>MNTIAWLGRLVIERIRGIGVAALMLLQIIFSLPSAGGFGRFVYQMHRVGVMSLLIITVSGLFIGLVLGLQGYSILVNVGSESMLGTMVSLTLLRELAPVVAALLFAGRAGSALTAEIGSMKQSEQLASMEMIGVDPLKQIVSPRLWAGIVSLPMLTVIFAAIGIVGGKLVGVDFLGVDEGSFWSGMQNNVQFGHDVVNGIIKSIVFALLCTWIAVFQGYACDPTPEGIATAMTRTVVYSSLCVLGFDFVLTAVMFGGI[2x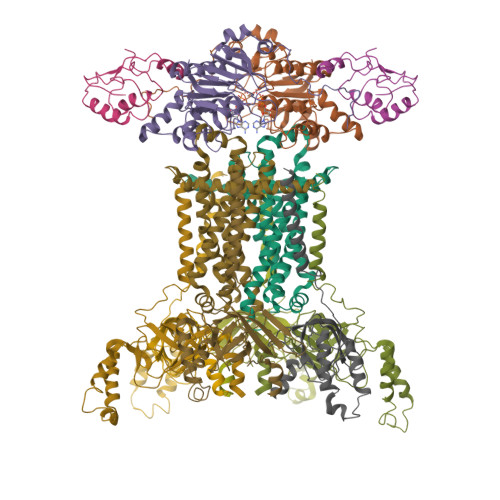];>MMNNKTPLSTQSLIEVKNLSFNRGERVIYDNISLNIRRGQITAIMGPSGTGKTTLLRLIGGQLVPDQGEVLLDGKDIAQMSRQELFAARARMGMLFQSGALFTDMSVYENVAFPIRAHTKLSENLIAELVALKLESVGLRGTEQLMPTELSGGMNRRVALARAIALDPDLIMYDEPFAGQDPIVKGVLTRLIRSLREALDLTTIIVSHDVPETLSIADYIYVVAEGKIQGEGTPEELQAYASPFVKQFLTGSAEGPVEYQFSHQAYLDNEVRP[2x];>[2x]VVQYLNQELVVSGKIDFENAEQQYQAGLAIIKKQTSFPLIVDLKQLEHGNTLALAVLVQWLRQTPQKSGLHFKNVPEKMLKIIQACHLQEDLHLVLEHHHHHH;>MKSRTSELAVGIFVIIFGIALFFLAMKVSGLVGTNLSDGYTMKAQFDNVNGLKPRAKVTMSGVTIGRVDSITLDPVTRLATVTFDLDGKLTSFNAEQLKEVQKNALDELRYSSDYTQATPAQQKTMEQQLISNMNSITSIDEDAYIMVATNGLLGEKYLKIVPGGGLNYLKRGDTISNTQGTMDLEDLISKFITGGGAGKVAAGSSSAEEKAPASTDSSAQPSFVE[6x]The most widespread of these mechanisms employs a “controller” (C) protein encoded by a gene downstream of its own promoter, and usually co-transcribed with the endonuclease (R) gene as a single transcriptional unit. The C-protein binds at various sites within the C/R promoter to regulate transcription of its own gene and the associated endonuclease gene. Unusually, in the RM system Esp1396I, the C-protein also represses the MTase (M) gene by binding to the promoter at the transcriptional start site, denoted OM where the C/R genes and the M gene are transcribed convergently from different promoters. Flexibility in this loop is very important for DNA sequence recognition, as it has been observed in the nucleoprotein structures to adopt different conformations depending on which operator site the protein is bound to.

The KD for the S52A interaction with the OM operator was 5 fold higher than the wild type, confirming the importance of this hydrogen bond interaction in stabilising the DNA-protein complex. Comparing ΔGs for S52A and WT, we obtain ΔΔG of 4.0 kJ mol−1, comparable with that for the Y37F mutant (3.1 kJ mol−1), and indeed in the crystal structure of the protein-DNA complex, both of these residues form a hydrogen bond to the phosphodiester backbone of the DNA. Five of the monomers in the asymmetric unit are observed to be in loop conformation I but the sixth more closely resembles that of conformation II, which is almost identical to that in the DNA-protein complex with the 19OM operator site. Both of the R46A crystal structures and the S52A crystal structure have adopted loop conformation III, despite the varying buffer conditions and crystallographic interactions in those three structures. The SO4 based interaction observed in the high-resolution wild type structure is also observed in the Y37A, S52A and monoclinic R46A structures. Both the monoclinic R46A and S52A structures show almost identical crystal contacts to those of the triclinic wild type protein, even though the space group and unit cell are different.

>GSHMESFLLSKVSFVIKKIRLEKGMTQEDLAYKSNLDRTYISGIERNSRNLTIKALELIMKGLEVSDVVFFEMLIKEILKHD[2x]>SEQNNAVLPKGVTQGEFNKAVQKFRALLGDDNVLVESDQLVPYNKIMMPVENAAHAPSAAVTATTVEQVQGVVKICNEHKIPIWTISTGRNFGYGSAAPVQRGQVILDLKKMNKIIKIDPEMCYALVEPGVTFGQMYDYIQENNLPVMLSFSAPSAIAGPVGNTMDRGVGYTPYGEHFMMQCGMEVVLANGDVYRTGMGGVPGSNTWQIFKWGYGPTLDGMFTQANYGICTKMGFWLMPK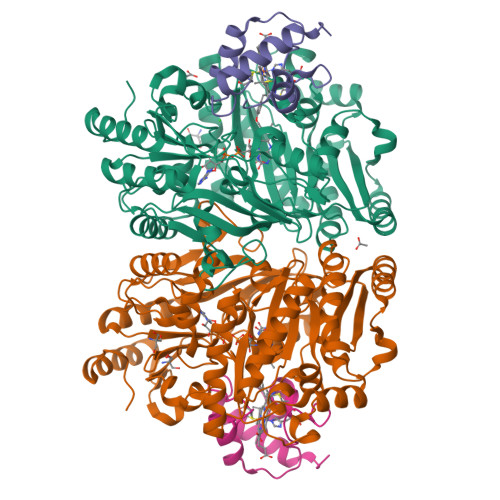PPVFKPFEVIFEDEADIVEIVDALRPLRMSNTIPNSVVIASTLWEAGSAHLTRAQYTTEPGHTPDSVIKQMQKDTGMGAWNLYAALYGTQEQVDVNWKIVTDVFKKLGKGRIVTQEEAGDTQPFKYRAQLMSGVPNLQEFGLYNWRGGGGSMWFAPVSEARGSECKKQAAMAKRVLHKYGLDYVAEFIVAPRDMHHVIDVLYDRTNPEETKRADACFNELLDEFEKEGYAVYRVNTRFQDRVAQSYGPVKRKLEHAIKRAVDPNNILAPGRSGIDLNNDF[2x];>DSQWGSGKNLYDKVCGHCHKPEVGVGPVLEGRGLPEAYIKDIVRNGFRAMPAFPASYVDDESLTQVAEYLSSLPAPAAQP[2x]> MASMT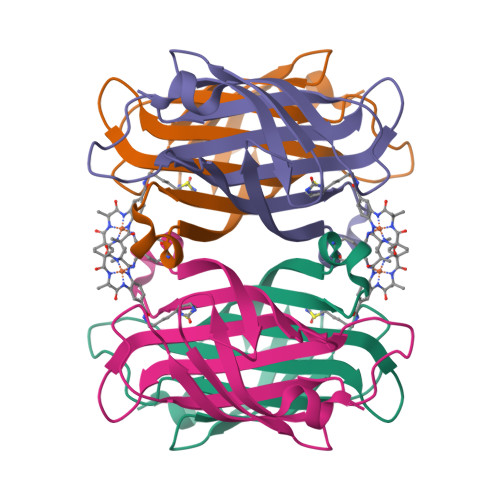GGQQMGRDQAGITGTWYNQLGSTFIVTAGADGALTGTYESAVGNAESRYVLTGRYDSAPATDGSGTALGWTVAWKNNYRNAHSATTWSGQYVGGAEARINTQWLLTRGTTEANAWKSTLVGHDTFTKVKPSAASIDAAKKAGVNNGNPLDAVQQ> GP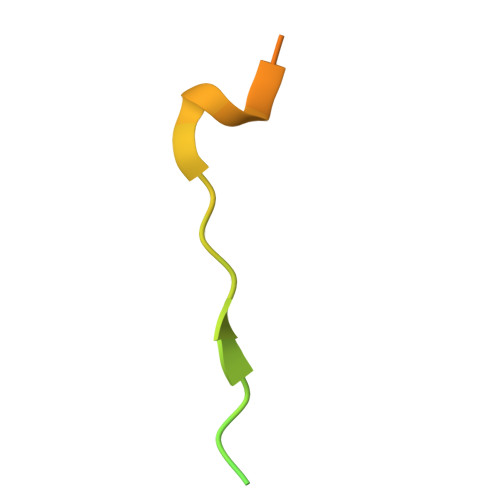GSDLDTEARDQPLNSKKKKRLLSFRDVDFEEDSDHLVQPCS>AEAGITGTWYAQLGDTFIVTAGADGALTGTYEAAVGDDDGDDDGDDDGAESRYVLTGRYDSAPATDGSGTALGWTVAWKNNYRNAHSATTWSGQYVGGAEARINTQWLLTSGTTEANAWKSTLVGHDTFTKVKPSAAS[2x];>AEAGITGTWYNQLGSTFIVTAGADGALTGTYESAVGNAESRYVLTGRYDSAPATDGSGTALGWTVAWKNNYRNAHSATTWSGQYVGGAEARINTQWLLTSGTTEANAWKSTLVGHDT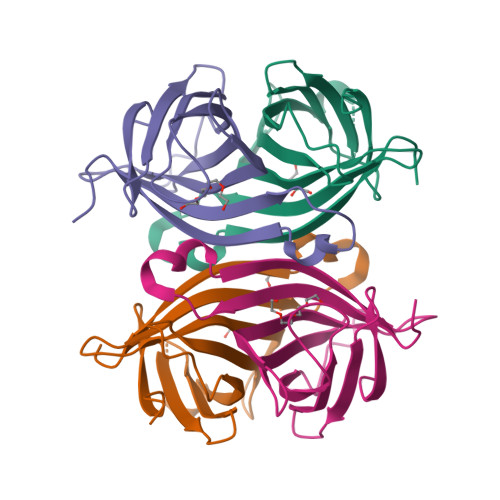FTKVKPSAAS[2x]A deazaflavin-dependent nitroreductase (Ddn) from Mycobacterium tuberculosis catalyzes the reduction of nitroimidazoles such as PA-824, resulting in intracellular release of lethal reactive nitrogen species. The N-terminal 30 residues of Ddn are functionally important but are flexible or access multiple conformations, preventing structural characterization of the full-length, enzymatically active enzyme. The split barrel-like fold is characterized by a central six-stranded antiparallel β barrel in a Greek key topology with four α helices: A at the N terminus (the putative helix removed for Ddn structure determination), B after an extended loop between strands β3 and β4, and C and D between strands β5 and β6. The identification of these residues and the lack of classic catalytic residues in the active site suggest that Ddn functions primarily by precisely orienting PA-824 for efficient direct hydride transfer from F420 and potentially through additional transition-state stabilization.

The full-length structure of a second, inactive homolog, nfa18080 from N. farcinica, was solved by X-ray crystallography in the presence of F420 (rmsd to Holo-1 is 1.1 Å over 109 aligned Cα atoms). The protein core, short N-terminal helix, and coenzyme binding site are conserved for nfa18080 relative to nfa33440. Electron density for the N terminus of nfa18080 starts at residue 5 and approaches the active site of a neighboring monomer in the crystal. The side chain of Y7 of one monomer stacks on top of the exposed Re face of F420 of another monomer at the location where one would expect the enzyme substrate to bind. The homolog structures provide insight into possible orientation of some conserved N-terminal residues in relation to the active site. However, because of low sequence homology (about 20% identity to Ddn residues 1–30) and flexibility of the N-terminal helix, these structures do not provide a reliable model for the missing Ddn N terminus.

>GMPLTGEYEPSPSDWARKQVETYENSGGTEGTTLQGKPVVVLTTKGAKTGKLRKTPLMRVEHNGEYAVVASLGGAPKHPVWYHNIKAEPHVELRDGTEVGDYTAREVTGEEKRVWWERAVEVWPDYAEYQTKTTREIPVFVLTPR[2x]> GPLGSMDPPTFTFNFNNEPWVRGRHETYLCYEVERMHNDTWVLLNQRRGFLCNQAPHKHGFLEGRHAELCFLDVIPFWKLDLDQDYRVTCFTSWSPCFSCAQEMAKFISKNKHVSLCIFTARIYDDQGRCQEGLRTLAEAGAKISIMTYSEFKHCWDTFVDHQGCPFQPWDGLD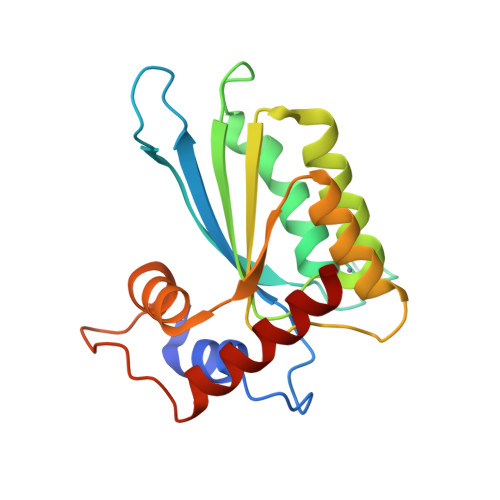EHSQDLSGRLRAILQ>[2x]ASQPPQVTVDKLKRLENDFGGRIGVYAIDTGSNKTFGYRANERFPLCSSFKGFLAAAVLSKSQQQEGLLNQRIRYDNRVMEPHSPVTEKQITTGMTVAELSAATLQYSDNGAANLLLEKLIGGPEGMTSFMRSIGDNVFRLDRWELELNSAIPGDDRDTSTPK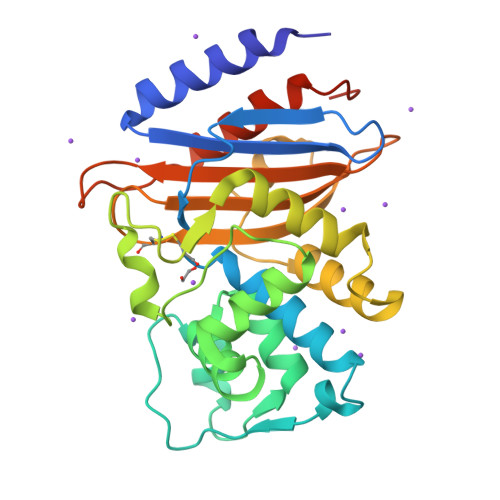AVAESMQKLAFGNVLGLTERHQLMDWFKGNTTGGARIRASVPANWVVGDKTGTCGVYGTANDYAVIWPVAHAPIVLAVYTSKPDRNSKHSDAVIADASRIVLESFNIDALRMATGKSIGF N^2^-[(2R)-2-{(1S)-1-[FORMYL(HYDROXY)AMINO]ETHYL}-5-PHENYLPENTANOYL]-N,3-DIMETHYL-L-VALINAMIDE 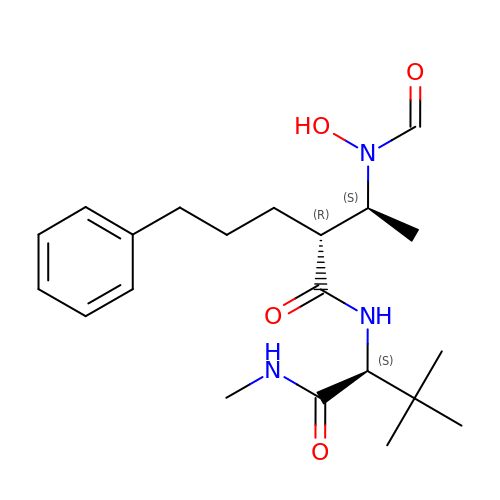| C21 H33 N3 O4 | GHVMTHKJUAOZJP-CGTJXYLNSA-N>QKEYMEYRPLGEEIERIRKGKNIPLRVFDENGVSSRSYQRFVQGNSELRISDLAIIVEILSISPMEMTEKLTPMSKTVLAKEQFNQAIFSKNFQESSRIVADYRAYYEKSSFALGKQEVMYSMLALEYLFNPQTVVTKEEIIALENQILERLINADVYTIFNLKFLALQKNVGLQPFPTSLLFRVLQSVNEREIIDIRSLEIIEQVIIDFLFAAIVSQNVPHILHVLSMFKEYEVGENNWRMILWKKIAEKIEMILTNEEIFADWSIFKEQILLSITLFLPKAKQEFFAGQLEKIEDSLKE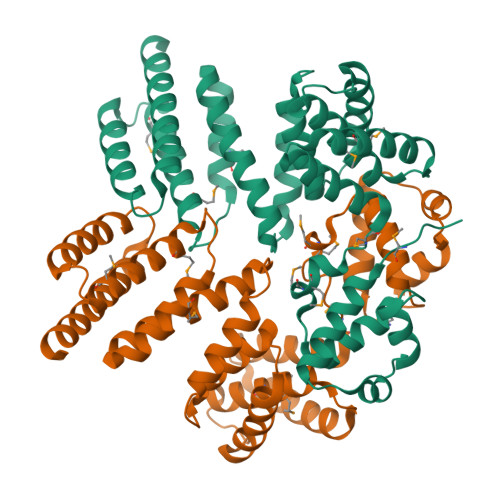IKENG[4x]> MHHHHHHGENLYFQGSGVEVIFYLSDREPLRLGSGEYTAEELCIRAAQACRISPLCHNLFALYDENTKLWYAPNRTITVDDKMSLRLHYRMRFYFTNWHGTNDNEQSVWRHSPKKQKNGYEKKKIPDATPLLDASSLEYLFAQGQYDLVKCLAPIRDPKTEQDGHDIENECLGMAVLAISHYAMMKKMQLPELPKDISYKRYIPETLNKSIRQRNLLTRMRINNVFKDFLKEFNNKTICDSSVSTHDLKVKYLATLETLTKHYGAEIFETSMLLISSENEMNWFHSNDGGNVLYYEVMVTGNLGIQWRHKPNVVSVEKEKNKLKRKKLENKDKKDEEKNKIREEWNNFSFFPEITHIVIKESVVSINKQDNKKMELKLSSHEEALSFVSLVDGYFRLTADAHHYLCTDVAPPLIVHNIQNGCHGPICTEYAINK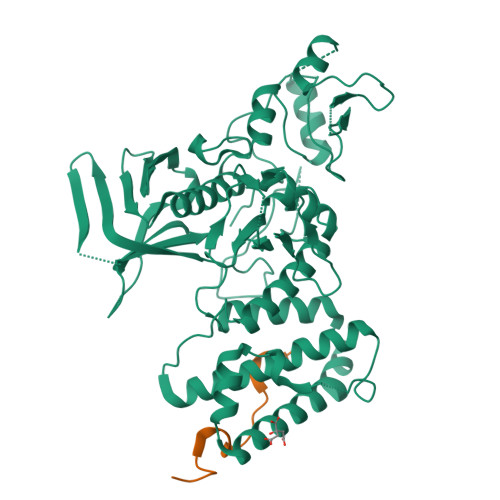LRQEGSEEGMYVLRWSCTDFDNILMTVTCFEKSEQVQGAQKQFKNFQIEVQKGRYSLHGSDRSFPSLGDLMSHLKKQILRTDNISFMLKRCCQPKPREISNLLVATKGNS;> GSKTLMGNPWFQRAKMPRALDFSGHTHPVATFQPSRPESVNDLFLCPQKELTGNS N~2~-[2-(5-chloro-1H-pyrrolo[2,3-b]pyridin-3-yl)-5-fluoropyrimidin-4-yl]-2-methyl-N-(2,2,2-trifluoroethyl)-D-alaninamide 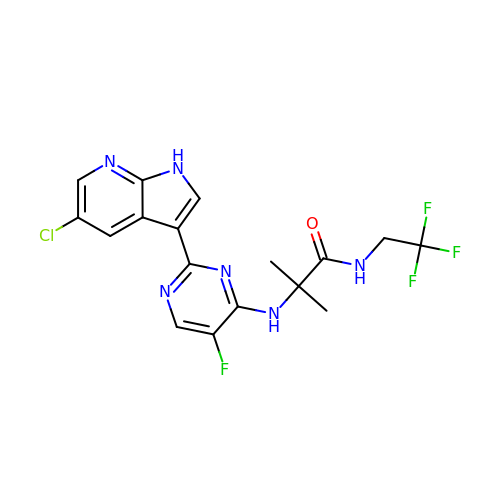| C17 H15 Cl F4 N6 O | GKLOLJGCCXEOJW-UHFFFAOYSA-N> MHHHHHHLPNITILATGGDIAGGGDSATKSNYTVGKVGVENLVNAVPQLKDIANVKGEQVVNIGSQDMNDNVWLTLAKKINTDCDKTDGFVITHGTDTMEETAYFLDLTVKCDKPVVMV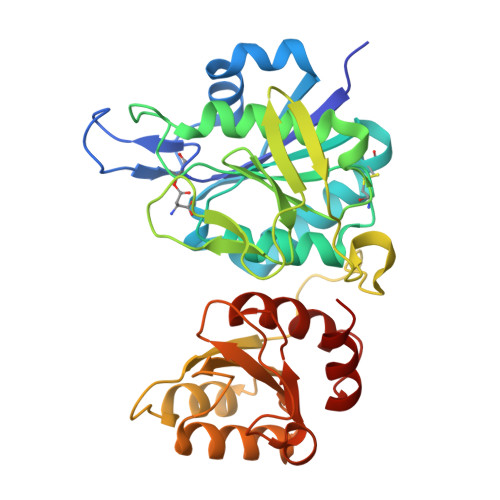GAMRPSTSMSADGPFNLYNAVVTAADKASANRGVLVVMNDTVLDGRDVTMTNTTDVATFKSVNYGPLGYIHNGKIDYQRTPARKHTSDTPFDVSKLNELPKVGIVYNYANASDLPAKALVDAGYDGIVSAGVGNGNLYKSVFDTLATAAKTGTAVVRSSRVPTGATTQDAEVDDAKYGFVASGTLNPQKARVLLQLALTQTKDPQQIQQIFNQY> MIPPRFEYHAPKSVGEAVALLGQ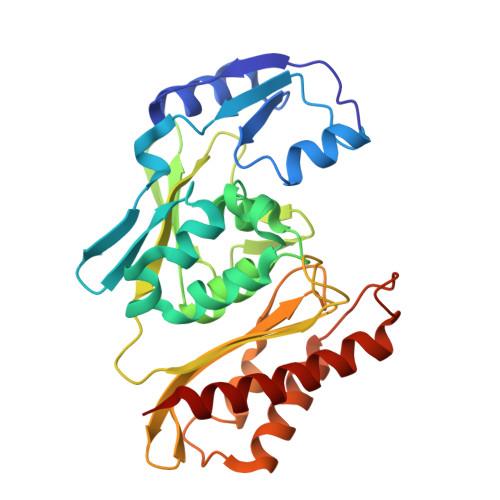LGSDAKLLAGGHSLLPMMKLRFAQPEHLIDINRIPELRGIREEGSTVVIGAMTVENDLISSPIVQARLPLLAEAAKLIADPQVRNRGTIGGDIAHGDPGNDHPALSIAVEAHFVLEGPNGRRTVPADGFFLGTYMTLLEENEVMVEIRVPAFAAGTGWAYEKLKRKTGDWATAGCAVVMRKSGGTVSHIRIALTNVAPTALRAEAAEAALLGKAFTKEAVQAAADAAIAICEPAEDLRGDADYKTAMAGQMVKRALNAAWARCA> ASMQKLINSVQNYAWGSKTALTELYGIANPQQQPMAELWMGAHPKSSSRITTANGETV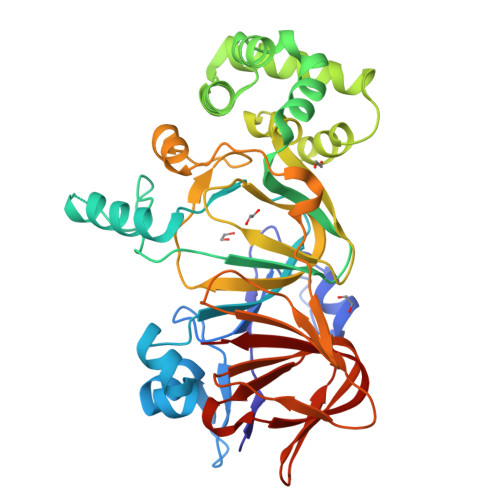SLRDAIEKNKTAMLGEAVANRFGELPFLFKVLCAAQPLSIQVQPNKRNSEIGFAKENAAGIPMDAAERNYKDPNHKPELVFALTPFLAMNAFREFSDIVSLLQPVAGAHSAIAHFLQVPNAERLSQLFASLLNMQGEEKSRALAVLKAALNSQQGEPWQTIRVISEYYPDDSGLFSPLLLNVVKLNPGEAMFLFAETPHAYLQGVALEVMANSDNVLRAGLTPKYIDIPELVANVKFEPKPAGELLTAPVKSGAELDFPIPVDDFAFSLHDLALQETSIGQHSAAILFCVEGEAVLRKDEQRLVLKPGESAFIGADESPVNASGTGRLARVYNKL>MPIVSKYSNERVEKIIQDLLDVLVKEEVTPDLALMCL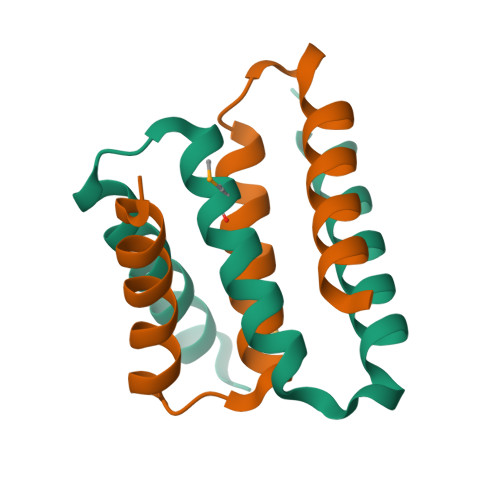GNAVTNIIAQVPESKRVAVVDNFTKALKQSVLEHHHHHH[2x]>[8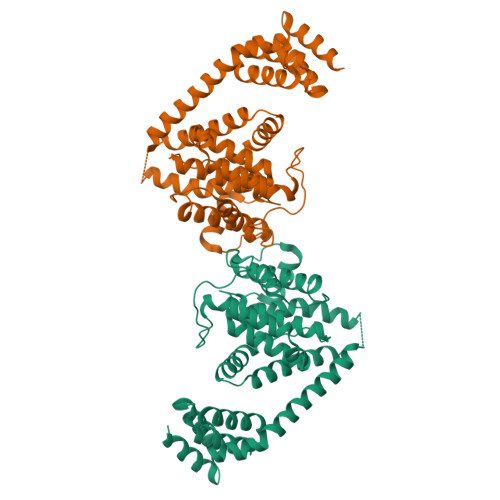x]GKLEARAALNQALEMKRQGKREKAQKLFMHALKMDPDFVDALTEFGIFSEEDKDIIQADYLYTRALTISPYHEKALVNRDRTLPLVEEIDQRYFSIIDSKVKKVMSIPKGNSALRRVMEETYYHHIYHTVAIEGNTLTLSEIRHILETRYAVPGKSLEEQNEVIGMHAAMKYINTTLVSRIGSVTISDVLEIHRRVLGYVDPVEAGRFRTTQVLVGHHIPPHPQDVEKQMQEFVQWLNSEEAMNLHPVEFAALAHYKLVYIHPFIDGNGRTSRLLMNLILMQAGYPPITIRKEQRSDYYHVLEAANEGDVRPFIRFIAKCTETTLDTLLFATTEYSVALPEAQP>NAAYQLLLSKETLNKILQYKQNLEKGLATPGKFFLEELSKQEKSISEMDITTFTQ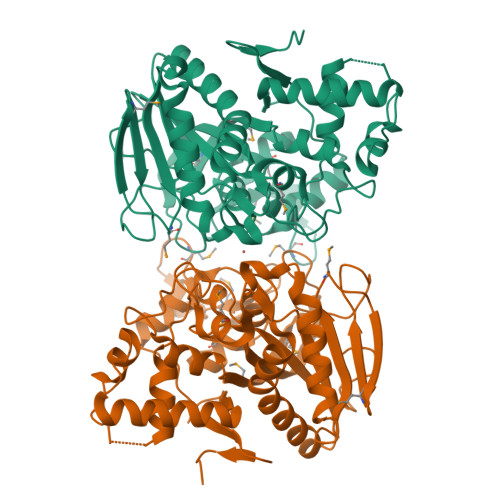LLIQSKKPQVFAESQVYHDGTDWTLEEESILGDVSVNMPVTMYNDGGHGSSFKNHPKPISGYLAYVPGALLASGSGPTSDMKEVLDNGKLNQDKLNALYERRLLPQLIHFNELARQNEKQAAITIPGIGTGCFSGAYYDVIKPYVRNALIHILEKHKDSLPYIDIIHYDPYMGDEPAEKKIGHMSFRVSPSGVVRGTTGQLDYPLGSNPDTHILVSIVAWDHFSWPGNDYWGGARQTDDGVKAASTDTMGQVTGATGVYDKKWGRYMPPESFTKDRKGMSDWGDYVRENGIVFNGPVLALDKSGKLDTLENVASRSSKAKVETTTTISDLVRSMFSLFSHS[3x]> TRIKITELNPHLMCVLCGGYFIDATT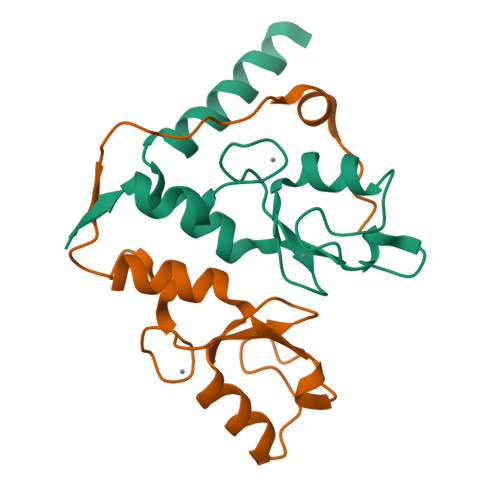IIECLHSFCKTCIVRYLETSKYCPICDVQVHKTRPLLNIRSDKTLQDIVYKLVPGLFKNEMKRRRDFYAAH;> KTWELSLYELQRTPQEAITDGLEIVVSPRSLHSELMCPICLDMLKNTMTTKECLHRFCADCIITALRSGNKECPTCRKKLVSKRSLRPDPNFDALISKIY> MPSPFQQTLLARAYHYVHPKTGRPIRQFRRYGDPRYINNEAALIRGQWGLITAD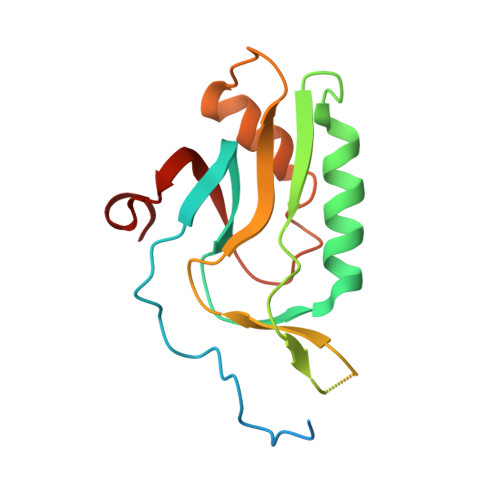FGMVTQSQMENARLAILRRLPRGSFTLTMHTDYEEFPVVKKSPESRMGAGKANIHHFAFKFTTGVPLFEIMPISARRLNQAEAEGIFLAGRPFIPLQTVVVPQGRVDEYHVFK>[4x]MRDVAIIGYGQTKFGELWEDSFRDLIVEAGVKAIKDANVDGGDIDAMYIGNMSGGLFVGQEHIASLIADHAGLNPVPCTRVEAACASGSLALRSAVLSVASGHHDVVLAGGVEKMTDVEDATAAIASASDQEWEAF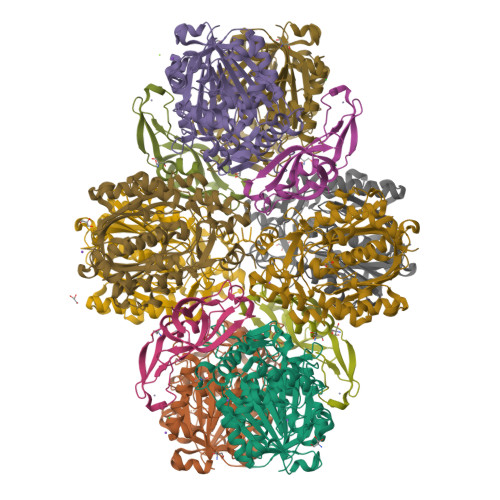FGATFPSLYAMMARRYMYQYGLTIEELSMWSVIAHENATKNKYAQFGFKTTLEQVMNASPVADPLTLMHCSPVSDGASALIVCDADKAEEFAPKDEIIYIKASTQASDTIALHDREDMTTLNAAKVASEKAYKLAKIAPEKIDVAEVHDCFAINGLILVEDLGFCKKGDAGKVIDEGKIRIDYDDFVTVNPSGGLKAAGHALGATGIRQVGELYWQLKQDKECKDRQATIKNGYGIAANVGGTGGTVCVHLLSDKR;>MVVRSWRHMKERYNLIGTRCKTCGKVYFPSRTVCPDCRRKGELEEFQLSGKGKIYTYSIVYAPPKEFNKLTPYVIAIVELEEGPKVTAQVDCDINKISIGIPVEAAFRRIKEDGKDGIISYGYKFVPITE[4x];>MKDIGIVGYGSYIPKYRIKVEEIAKVWGKDPEAIKKGLVVNEKSVPSPDEDTATIAVEAARNAVKRAGINAEKIGAVYVGSESHPYAVKPTSATVAEAIGATPDLTAADLEFACKAGTAGIQMCMGLVGSGLIEYGMAIGADTAQGAPGDALEYTASAGGAAYIIGNKKDEMIAVFNGTYSYTTDTPDFWRREGQSYPKHGGRFTGEPAYFKHVLNAAKGIMEKMGTTVKDYDYCVFHQPNGKFYIKAAKSLGFTNEQYKYGLLTPYLGNTYSGAVPLGLSNILDHAEEGARILAVSYGSGAGSDAFDITVTERIKEVVDKAPKTLDLLNRKKYIDYAVYVKYRGKIKI[4x]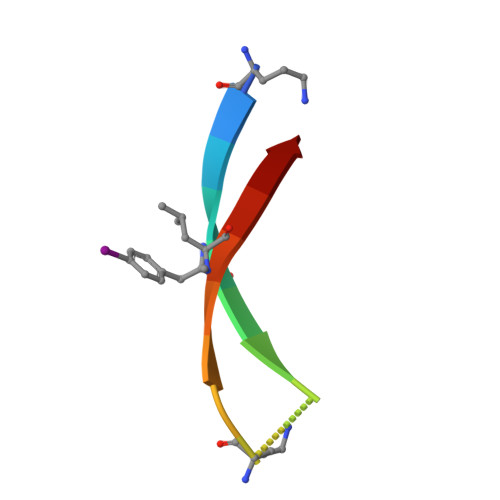> AYLLFYTEAKVALAVK> AAQLSEQLAELEKRSGGRLGVAVLDTATGRRIAYRGDERFPMCSTFKALLAAAVLARVDQGKERLDRRITYGKEDLVDYSPVTEKHVGDGMTVAELCEAAITLS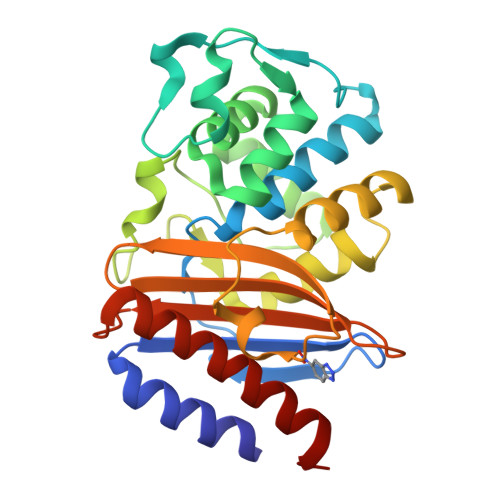DNTAANLLLEALGGPAALTAFLRSIGDEVTRLDRWEPELNEAAPGDPRDTTTPAAMAATLRTLLLGDALSPASRQQLVDWLVANKTGDKRLRAGLPADDRVGDKTGTGGHGTTNDIAVIWPPGRAPIVVTVYLTESQVDADARDAVIAEVGRLVVEAFHHHHHH The self-labeling protein tags (SLPs) HaloTag7, SNAP-tag, and CLIP-tag allow the covalent labeling of fusion proteins with synthetic molecules for applications in bioimaging and biotechnology. The three most popular SLPs are HaloTag7 (HT7),14 SNAP-tag (SNAP),15 and CLIP-tag (CLIP)16. To guide the selection of an SLP–substrate pair and provide guidelines for the design of substrates, we report a systematic and comparative study of the labeling kinetics and substrate specificities of HaloTag7, SNAP-tag, and CLIP-tag. We complement these kinetic studies by reporting crystal structures of HT7 and SNAP covalently labeled with rhodamine-based fluorophores, providing a detailed understanding of their substrate preferences.

HT7 was engineered from a bacterial dehalogenase (DhaA from Rhodococcus sp.), an enzyme that can hydrolyze halogenated alkanes. HT7 reacts specifically with chloroalkane-PEG (CA) molecules resulting in covalent bonding of the alkane chain to the reactive aspartate and release of a chloride ion. In addition to the conventional α/β-hydrolase topology, HT7 features an extra capping domain made of six α-helices (Hlx4–9) that partially cover the catalytic site and form an entry channel for the CA substrate. After reaction, the PEG-alkane ligand is buried in the protein, while the xanthene moiety of the dye lays on the distorted α-helix 8 (Hlx8) in a conformation partially constrained by the crystal packing. The alkane-fluorophore is positioned by the Hlx6–turn–Hlx7–turn–Hlx8 motif of the HT7 capping domain from which T172Hlx8 and, to a lesser extent, T148Hlx6 form hydrogen bonds with the oxygen and the nitrogen of the amide bond linking PEG-alkane and fluorophore. CA-TMR and CA-CPY have similar conformations in both structures with only minor differences in their torsion angles. In comparison to TMR, one of the additional methyl groups of CPY is forming van der Waals interactions at the protein surface, potentially explaining the increased affinity of CA-CPY relative to that of CA-TMR. The mechanism underlying the equilibrium shift from the spirocyclic nonfluorescent to the zwitterionic fluorescent form is not yet fully understood, but our results indicate that the planar, zwitterionic form of rhodamines (e.g., TMR and CPY) features energetically favorable interactions with the HT7 surface, thus potentially favoring this state of the fluorophore when attached to the protein.

>GIGTGFPFDPHYVEVLGERMHYVDVGPRDGTPVLFLHGNPTSSYVWRNIIPHVAPTHRCIAPDLIGMGKSDKPDLGYFFDDHVRFMDAFIEALGLEEVVLVIHDWGSALGFHWAKRNPERVKGIAFMEFIRPIPTWDEWPEFARETFQAFRTTDVGRKLIIDQNVFIEGTLPMGVVRPLTEVEMDHYREPFLNPVDREPLWRFPNELPIAGEPANIVALVEEYMDWLHQSPVPKLLFWGTPGVLIPPAEAARLAKSLPNCKAVDIGPGLNLLQEDNPDLIGSEIARWLSTLEI[5x]N-2-THIOPHEN-2-YL-ACETAMIDE BORONIC ACID | C7 H10 B N O3 S | 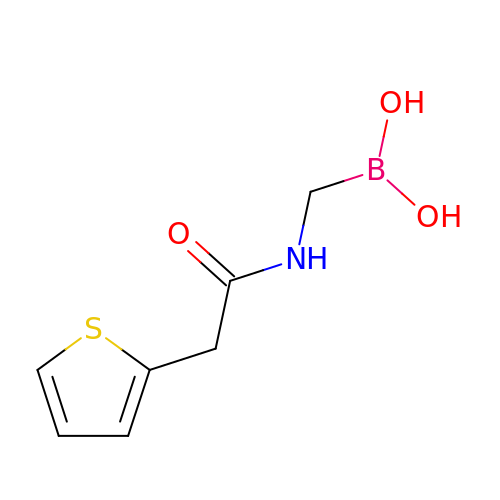VXAPSUDMBNWYNC-UHFFFAOYSA-N The U1A/U2B″/SNF family of RBPs is found in the U1 and/or U2 small nuclear ribonucleoprotein (snRNP) components of the spliceosome. Jawed vertebrates use U1A to bind stem-loop II of U1 snRNA (U1SLII) and U2B″ in conjunction with the leucine-rich repeat (LRR) protein U2A′ to bind SLIV of U2 snRNA (U2SLIV). Both U1A and U2B″ employ an N-terminal RNA recognition motif (RRM) to specifically recognize their RNA targets. Here, we report crystal structures of four states of dSNFRRM1 at 2 Å resolution or better: the free dSNFRRM1 (residues 1–96; dSNF1–96), dSNF1–96–dU1SLII, dU2A′–dSNF1–96, and dU2A′–dSNF1–96–dU2SLIV. Altogether with the characterization of dSNFRRM1 dynamics alone and in complexes by NMR spectroscopy and targeted mutagenesis combined with binding studies, we delineated how the intrinsic dSNFRRM1 RNA-binding capacity and specificity are fine-tuned by networks of intra-molecular interactions that modulate dSNFRRM1 dynamics, and how the auxiliary dU2A′ protein can capitalize on intrinsic dSNFRRM1 flexibility to gear dSNFRRM1 binding specifically to dU2SLIV.

We determined a crystal structure of dSNFRRM1 based on a construct containing residues 1–96 of dSNF (dSNF1–96) at 1.49 Å resolution, showing that the protein adopts a classic RRM fold, with Tyr10-Gln51-Phe53 displayed on the surface of its four-stranded anti-parallel β-sheet, in agreement with the previous NMR structure of dSNFRRM1 19. Comparison of the six crystallographically independent dSNF1–96 molecules indicated intrinsic conformational flexibility in the RNA-binding surface of dSNF1–96, predominantly affecting loop L3 (residues 42–51; Cα root-mean-square deviation (rmsd) 0.16–1.10 Å with a maximum displacement of 1.47 Å) and to a lesser extent L1 (residues 13–19; rmsd 0.10–0.14 Å with a maximum displacement of 0.21 Å), as well as side chain conformations in the Tyr-Gln-Phe motif. Furthermore, the conformations and positions of the N-terminal extensions (residues 1–7), which in one case forms an additional α-helix, and the C-terminal loops L6 (residues 84–87) and α3 helices (residues 88–94) differ among the six dSNF1–96 copies, in agreement with solution NMR data showing that the latter element undergoes extensive ps-ns motions.Fig. 1 dSNF1-96 structure and conformational flexibility. a Sequence alignment of dSNFRRM1, hU1ARRM1 and hU2B″RRM1. Truncating α3 at residue 96 causes the C-terminal region of the corresponding construct to become more flexible on the ns-ps and ms timescales as the helical structure is disrupted, consistent with three copies of dSNF1–96 in the crystal structure entirely lacking electron density for the α3 region. Only α2 residues exhibited no measurable exchange.

>GAMEMLPNQTIYINNLNEKIKKEELKKSLYAIFSQFGQILDIVALKTLKMRGQAFVIFKEIGSASNALRTMQGFPFYDKPMQIAYSKSDSDIVAKIKG[6x]> VEFNTDVLDAADKKNIDFTRFSEAGYVLPGXX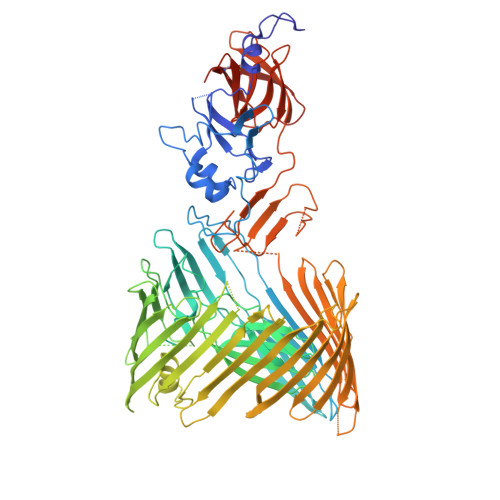XXXXXXXXXXXXXXXXXXXXXXXXXXXXXXXXXXXXXXXXXXXXXXXXXXXXXXXXXXXXXXXXXXXXXXXXXXXXXXXXXXXXXXXXXLPPSRWDDGIPGLMLDYNLNGTVSRNYQGGDSHQFSYNGTVGGNLGPWRLRADYQGSQEQSRYNGEKTTNRNFTWSRFYLFRAIPRWRANLTLGENNINSDIFRSWSYTGASLESDDRMLPPRLRGYAPQITGIAETNARVVVSQQGRVLYDSMVPAGPFSIQDLDSSVRGRLDVEVIEQNGRKKTFQVDTASVPYLTRPGQVRYKLVSGRSRGYGHETEGPVFATGEASWGLSNQWSLYGGAVLAGDYNALAAGAGWDLGVPGTLSADITQSVARIEGERTFQGKSWRLSYSKRFDNADADITFAGYRFSERNYMTMEQYLNARYRNDYSSREKEMYTVTLNKNVADWNTSFNLQYSRQTYWDIRKTDYYTVSVNRYFNVFGLQGVAVGLSASRSKYLGRDNDSAYLRISVPLGTGTASYSGSMSNDRYVNMAGYTDTFNDGLDSYSLNAGLNSGGGLTSQRQINAYYSHRSPLANLSANIASLQKGYTSFGVSASGGAXXXXXXXXXXXXXXXXXXXXXXXXXXXXXXXXXXXXXXXXXXGKRLFAILRLADGSQPPFGASVTSEKGRELGMVADEGLAWLSGVTPGETLSVNWDGKIQCQVNVPETAISDQQLLLPCTPQKLVPRGSHHHHHH> SMDMPVERILEAELAVEPKTETYVEANMGLNPSSPN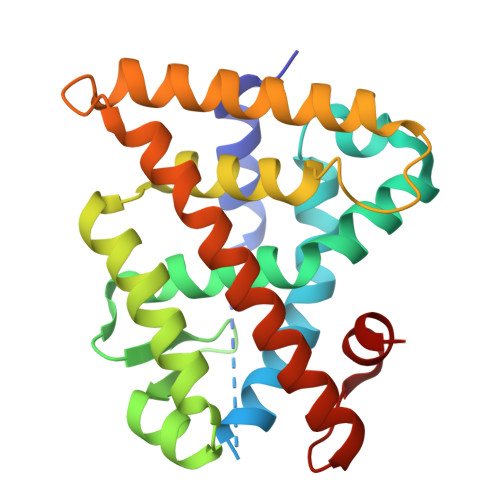DPVTNICQAADKQLFTLVEWAKRIPHFSELPLDDQVILLRAGWNELLIASFSHRSIAVKDGILLATGLHVHRNSAHSAGVGAIFDRVLTELVSKMRDMQMDKTELGCLRAIVLFNPDSKGLSNPAEVEALREKVYASLEAYCKHKYPEQPGRFAKLLLRLPALRSIGLKCLEHLFFFKLIGDTPIDTFLMEMLE> MASSGADSGEIILFSGSNHADFKAW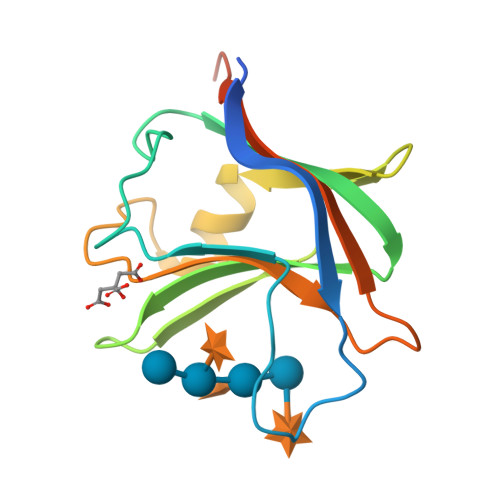GGDDWPSAFEISPKYEPMKLDLNKNFEIKVDYNGADIVLIFARWDKDIWAQISPYYVVDGTAVFTKEQIAKAYGSDDFSGLDYIAVKPLPSEEGVTVTKVSGIYTNGGSEDLEHHHHHH>[4x]GPLGSPEFMADRQPYMTNGIQAAVVEWIRALDLEIISLLLSRAWPMALLATSELRWRPTVLTDTDNVVRLDRRQRLVRWDRRPPNEIFLDGFVPIVTRENPDWEETDLYGFAKNNHPSIFVSTTKTQRNKKKYVWTPRNANRGIVY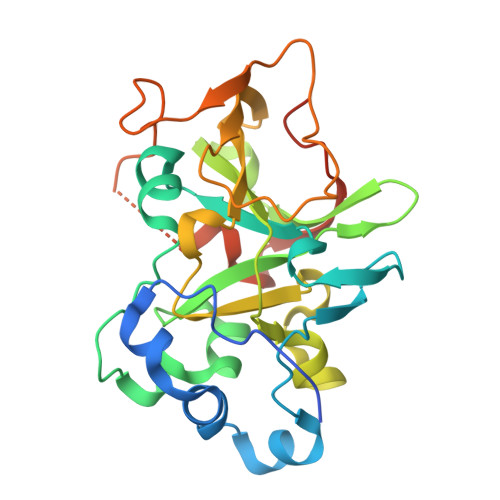QYEIYAPGGVDVNDSFSDASPWPNQMQVAFPGGIQNIYIRSARELHNGRIQRIWINPNFLDPGDLEPIVSSSRTPQVIWRMNHPDGGHRDQRSERSASSYDDLMYGGTGNVQEDTFGDEPNNPKPIAAG> MPRYQATLLIELKKGILDPQGRAVEGVLKDLGHPVEEVRVGKVLEIVFPAENLLEAEEKAKAMGALLANPVMEVYALEALKEL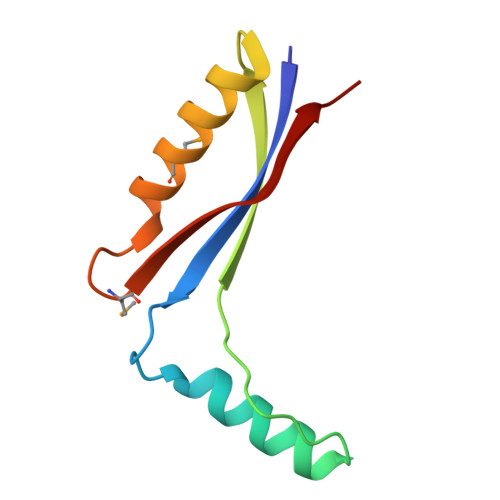P>[2x]XGEI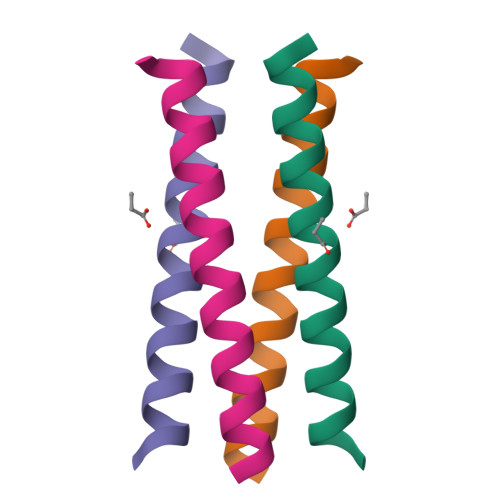KQQLAEIKQQLAEIKWQLAEIKQQLAGX> GPDDHMKKRQRFVDKNGRCNVQHGNLGSERAETLMFSEHAVISMRDGKLTLMFRVGNLRNSHMVSAQIRCKLLKSRQTPEGEFLPLDQLELDVGASTGADQLFLVSPLTICHVIDAKSPFYDLSQRSMQTEQFE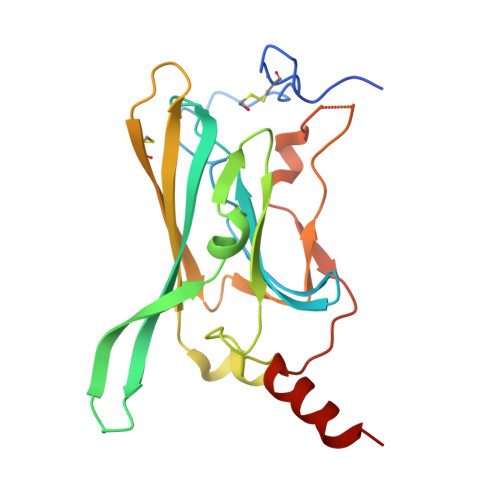VVVILEGIVETTGMTCQARTSYTEDEVLWGHRFFPVISLEEGFFKVDYSQFHATFEVPTPPYSVKEQEEMLLMSSP> MAFGRTRPTLSSPLVPVWNDLRALQVFTSQEYMQKRGPGFTNTLEYKLSCLNPV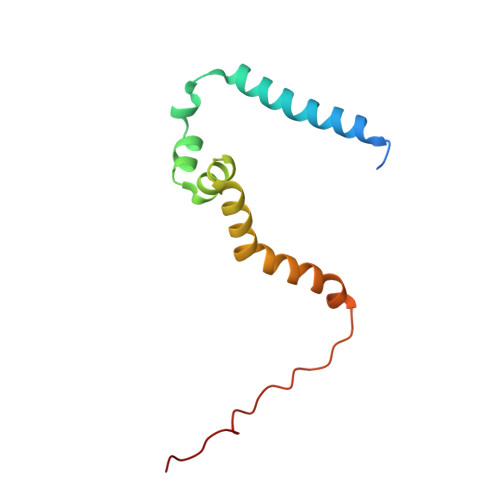KWYDMMKVMPGGKAFVGTALGLALFGGWGVEFVKNISVMTKEKPPIDWNNEKLGHLTRS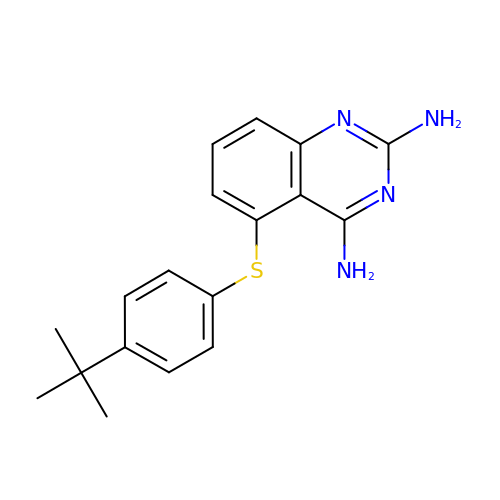5-[4-TERT-BUTYLPHENYLSULFANYL]-2,4-QUINAZOLINEDIAMINE | C18 H20 N4 S | MNYDVPDMLAJJPB-UHFFFAOYSA-N>[2x]MGSSHHHHHHSSGENLYFQGHMAAPFDKSRNVAQSIDQLIGQTPALYLNKLNNTKAKVVLKMECENPMASVKDRLGFAIYDKAEKEGKLIPGKSVVVESSSGNTGVSLAHLGAIRGYKVIITMPESMSLERRCLLRIFGAEVILTPAALGMKGAVTMAKKIVTANPNAVLADQFATKYNALIHEETTGPEIWEQTNHNVDCFIAGVGTGGTLTGVARALKKMGSHARIVAVEPMESPVLSGGKPGAHKIQGIGPGFVPDVLDRSLIDEVFCVAGDDAIETALKLTRSDGVFCGFSGGANVYAALKIAERPEMEGKTIVTIIPSFGERYLSTALYRSVRDEVSSLPVVDASELQD;> EEEEE;> EEEE

Leishmania, a widespread and important protozoan pathogen of humans and animals, requires cysteine for protein biosynthesis and as a precursor of trypanothione, a glutathione–spermidine conjugate unique to trypanosomatids with an essential role in redox metabolism and antioxidant defence. The parasite can also produce cysteine from serine in a two-step process. Firstly, serine acetyltransferase (SAT) generates O-acetylserine (OAS) to supply the substrate for the second stage, which is catalyzed by the pyridoxal phosphate (PLP)-dependent cysteine synthase (CS; EC 2.5.1.47). This de novo pathway for cysteine biosynthesis is found in plants, bacteria and some protozoa, but is absent from mammals.

The structure of LmCS was determined to a resolution of 1.8 Å. The biologically active unit, a dimer, constitutes the asymmetric unit. A surface loop from residues 214 to 241 is disordered and is therefore missing from the model. The LmCS subunit contains two domains. In addition, residues 307–333 at the C-terminus form an extended helix–loop–helix structure that stretches across the surface of the partner subunit. However, the crystals were colourless and there was no electron density to indicate that PLP was present. A fragment of the crystallization agent PGA-LM is bound in an ordered fashion to the same region of both subunits of the LmCS dimer. The interactions between carboxyls from PGA and the side chain and main chain of Thr83 and the main-chain amides of Asn82, Ser274 and Phe273 are common to both binding sites. The binding of PGA may have contributed to the absence of PLP and the unresolved loop between residues 214 and 241 in LmCS. In LmCS, the placement of these two residues ensures that the active site is considerably widened with respect to that found in orthologues of known structure.> MAFEALTGINGDLITRSWSASKQAYLTERYHKEEAGAVVIFAFQPSFSEKDFFDPDNKSSFGEIKLNRVQFPCMRKIGKGDVATVNEAFLKNLEAIIDPRTSFQASVEMAVRSRKQIVFTGHSSGGATAILATVWYLEKYFIRNPNVYLEPRCVTFGAPLVGDSIFSHALGREKWSRFFVNFVSRFDIVPRIMLARKASVEETLPHVLAQLDPRKSSVQESEQRITEFYTRVMRDTSTVANQAVCELTGSAEAFLETLSSFLELSP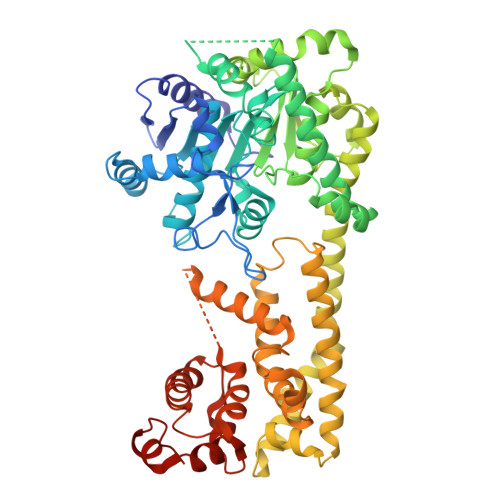YRPAGTFVFSTEKRLVAVNNSDAILQMLFYTSQASDEQEWSLIPFRSIRDHHSYEELVQSMGKKLFNHLDGENSIESTLNDLGVSTRGRQYVQAALEEEKKRVENQKKIIQVIEQERFLKKLAWIEDEYKPKCQAHKNGYYDSFKVSNEENDFKANVKRAELAGVFDEVLGLMKKCQLPDEFEGDIDWIKLATRYRRLVEPLDIANYHRHLKNEDTGPYMKRGRPTRYIYAQRGYEHYILKPNGMIAEDVFWNKVNGLNLGLQLEEIQETLKNSGSECGSCFWAEVEELKGKPYEEVEVRVKTLEGMLGEWITDGEVDDKEIFLEGSTFRKWWITLPKNHKSHSPLRDYMMDEITDT>MGSSHHHHHHENLYFQGCGPNRSKEDIDKALNKDNSKDKPNQLTMWVDGDKQMAFYKKITDQYTKKTGIKVKLVNIGQNDQLENISLDAPAGKGPDIFFLAHDNTGSAYLQGLAAEIKLSKDELKGFNKQALKAMNYDNKQLALPAIVETTALFYNKKLVKNAPQTLEEVEANAAKLTDSKKKQYGMLFDAKNFYFNYPFLFGNDDYIFKKNGSEYDIHQLGLNSKHVVKNAERLQKWYDKGYLPKAATHDVMIGLFKEGKVGQFVTGPWNINEYQETFGKDLGVTTLPTDGGKPMKPFLGVRGWYLSEYSKHKYWAKDLMLYITSKDTLQKYTDEMSEITGRVDVKSSNPNLKVFEKQARHAEPMPNIPEMRQVWE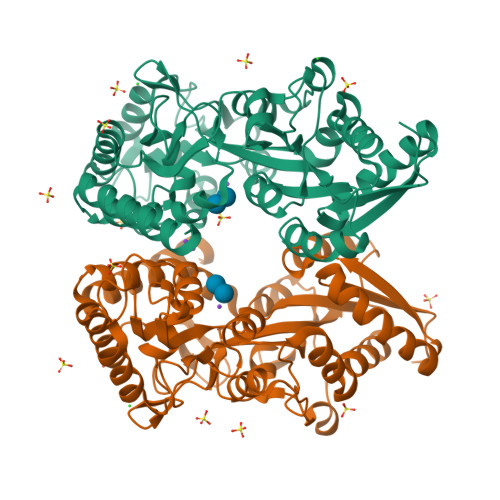PMGNASIFISNGKNPKQALDEATNDITQNIKILHPSQNDKKGD[2x]N-[5-(3,5-DIFLUOROBENZYL)-1H-INDAZOL-3-YL]-2-[(4-HYDROXYCYCLOHEXYL)AMINO]-4-(4-METHYLPIPERAZIN-1-YL) BENZAMIDE | C32 H36 F2 N6 O2 | 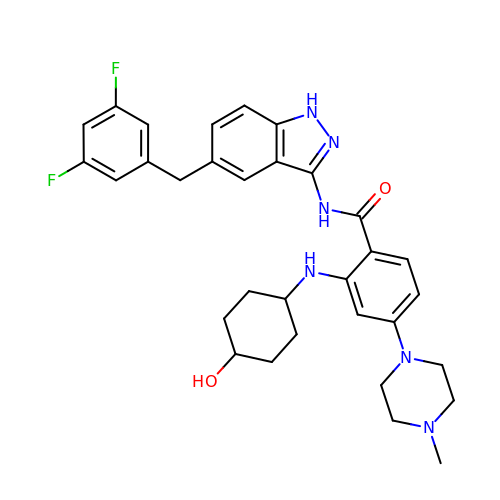COPINYWCESNOFK-YOCNBXQISA-N> SPNSQYLKTRILDIYTPEQRAGIEKSEDWRQFSRRMDTHFPKLMNELDSVYGNNEALLPMLEMLLAQAWQSYSQRNSSLKDIDIARENNPDWILSNKQVGGVCYVDLFAGDLKGLKDKIPYFQELGLTYLHLMPLFKCPEGKSDGGYAVSSYRDVNPALGTIGDLREVIAALHEAGISAVVDFIFNHTSNEHEWAQRCAAGDPLFDNFYYIFPDRRMPDQYDRTLREIFPDQHPGGFSQLEDGRWVWTTFNSFQWDLNYSNPWVFRAMAGEMLFLANLGVDILRMDAVPIIWKQMGTSCENLPQAHALIRAFNAVMRIAAPAVFFKSEAIVHPDQVVQYIGQDECQIGYNPLQMALLWNTLATREVNLLHQALTYRHNLPEHTAWVNYVRSHDDIGWTFADEDAAYLGISGYDHRQFLNRFFVNRFDGSFARGVPFQYNPSTGDCRVSGTAAALVGLAQDDPHAVDRIKLLYSIALSTGGLPLIYLGDEVGTLNDDDWSQDSNKSDDSRWAHRPRYNEALYAQRNDPSTAAGQIYQDLRHMIAVRQSNPRFDGGRLVTFNTNNKHIIGYIRNNALLAFGNFSEYPQ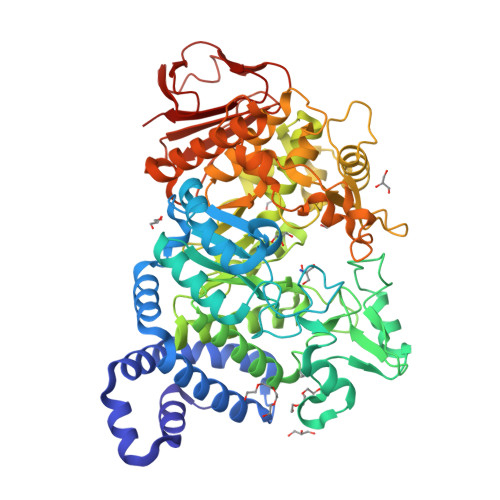TVTAHTLQAMPFKAHDLIGGKTVSLNQDLTLQPYQVMWLEIA>MSKSVFVGELTWKEYEARVAAGDCVLMLPVGALEQHGHHMCMNVDVLLPTAVCKRVAERIGALVMPGLQYGYKSQQKSGGGNHFPGTTSLDGATLTGTVQDIIRELARHGARRLVLMNGHYEN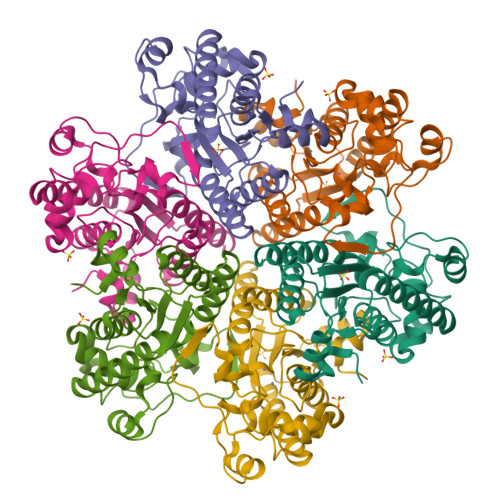SMFIVEGIDLALRELRYAGIQDFKVVVLSYWDFVKDPAVIQQLYPEGFLGWDIEHGGVFETSLMLALYPDLVDLDRVVDHPPATFPPYDVFPVDPARTPAPGTLSSAKTASREKGELILEVCVQGIADAIREEFPPT[6x]3-chloranyl-4-[1-[(1~{R})-1-[5-[3-chloranyl-2-fluoranyl-6-(1,2,3,4-tetrazol-1-yl)phenyl]-1-oxidanyl-pyridin-2-yl]-2-cyclopropyl-ethyl]pyrazol-4-yl]-5-fluoranyl-pyridine 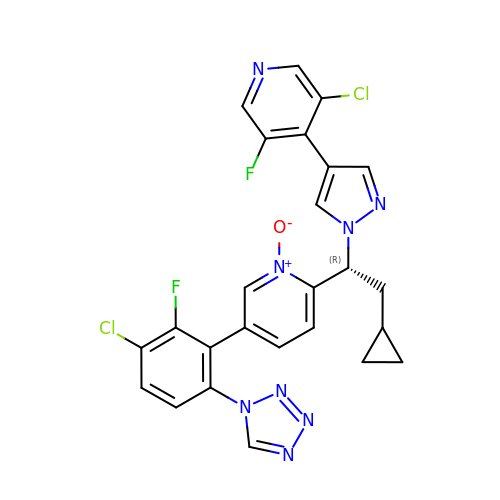| C25 H18 Cl2 F2 N8 O | HHZXBCQTDGQCBH-JOCHJYFZSA-N> MDSGYSSSYAAAAGMHVVICPWLAFGHLLPCLDLAQRLASRGHRVSFVSTPRNISRLPPVRPALAPLVAFVALPLPRVEGLPDGAESTNDVPHDRPDMVELHRRAFDGLAAPFSEFLGTACADWVIVDVFHHWAAAAALEHKVPCAMMLLGSAHMIASIADRRLERAETESPAAAGQGRPAAAPTFEVARMKLIRTKGSSGMSLAERFSLTLSRSSLVVGRSCVEFEPETVPLLSTLRGKPITFLGLMPPLHEGRREDGEDATVRWLDAQPAKSVVYVALGSEVPLGVEKVHELALGLELAGTRFLWALRKPTGVSDADLLPAGFEERTRGRGVVATRWVPQMSILAHAAVGAFLTHCGWNSTIEGLMFGHPLIMLPIFGDQGPNARLIEAKNAGLQVARNDGDGSFDREGVAAAIRAVAVEEESSKVFQAKAKKLQEIVADMACHERYIDGFIQQLRSYKDLEHHHHHH

Here, we report the biochemical and structural characterization of OsUGT91C1, a glycosyltransferase from Oryza sativa, which is efficient at catalyzing β (1–2) glucosylation. OsUGT91C1 is able to catalyze the addition of both glucose 2-1-R1 and glucose 2-1-R2 with roughly equal efficiency. It also catalyzes a third reaction, β (1–6) glucose addition, to create previously uncharacterized compounds. The enzyme’s ability to bind steviol glycoside substrate in three modes underlies its flexibility to catalyze β (1–2) glucosylation in two distinct orientations as well as β (1–6) glucosylation.

We chose STB, which lacks the R2 glycan, as a means to obtain a complex with the R1 end at the catalytic site. We could build both glucose 1-R1 and glucose 2-1-R1 into the electron density at the active site. Compared to the complexes with the R2 end at the catalytic site, the steviol aglycone of STB has undergone a 180° rotation to swap the R1 and R2 ends. The position and volume occupied by the steviol aglycone in this rotated arrangement are very similar to those complexes with R2 glycans at the catalytic site. In addition to steviol aglycone rotation, glucose 1-R1 of STB undergoes a 180° flip around the glycosidic bond to the aglycone. As a result of the flip, it is 6-hydroxyl, not 2-hydroxyl of glucose 1-R1, hydrogen-bonded to His27. In this orientation, glucose 1-R1 does not form a bidentate hydrogen bond with Glu283 but retains the hydrogen bonds of the 4-hydroxyl with Glu283 and Trp22. Glucose 2-1-R1 is found in a previously undisclosed pocket where it makes contact with His93, and its hydrophobic face stacks against the aromatic ring of Phe379. We believe that these interactions with glucose 2-1-R1 stabilize the flipped arrangement of glucose 1-R1. Guided by structure, we constructed three mutants H93A, H93W, and F379A, to suppress β (1–6) glucosylation by eliminating the cryptic glucose pocket seen for glucose 2-1-R1 in the STB complex.>[2x]GSDELYRQSLE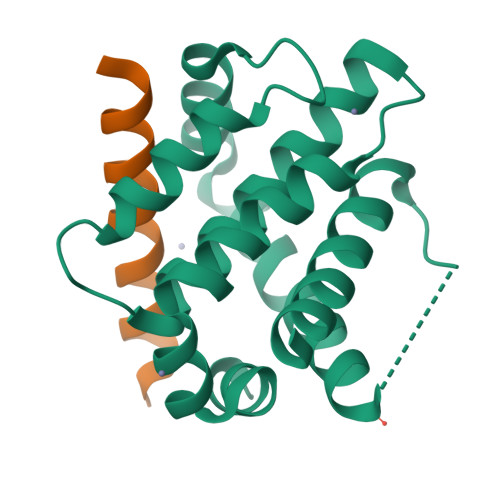IISRYLREQATGAKDTKPMGRSGATSRKALETLRRVGDGVQRNHETAFQGMLRKLDIKNEDDVKSLSRVMIHVFSDGVTNWGRIVTLISFGAFVAKHLKTINQESCIEPLAESITDVLVRTKRDWLVKQRGWDGFVEFFHVEDLEGG;>[2x]RPEIWAAQEIRRIGDENNAYYAR> AEAGIT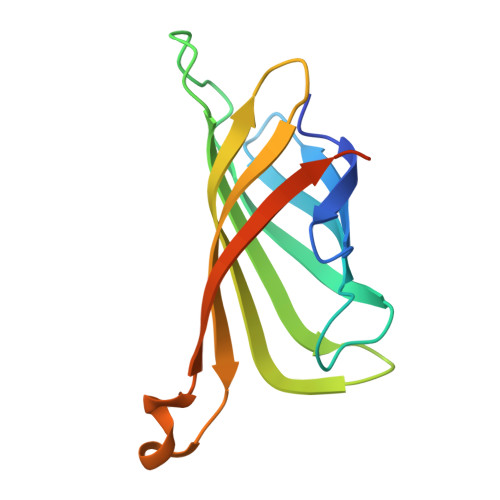GTWYNQLGSTFIVTAGADGALTGTYESAVGNAESRYVLTGRYDSAPATDGSGTALGWTVAWKNNYRNAHSATTWSGQYVGGAEARINTQWLLTSGTTEANAWKSTLVGHDTFTKVKPSAASEEEEEE>[8x]SLGTCLLPEVTEEDQGRICVVIDLDETLVHSSFKPINNADFIVPIEIEGTTHQVYVLKRPYVDEFLRRMGELFECVLFTASLAKYADPVTDLLDRCGVFRARLFRE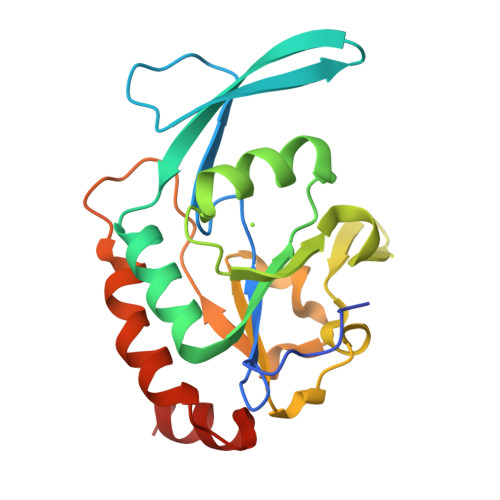SCVFHQGCYVKDLSRLGRDLRKTLILDNSPASYIFHPENAVPVQSWFDDMADTELLNLIPIFEELSGAEDVYTSLGQLRAP>[4x]MGRELSFFLQKESAGFFLGMDAPAGSSVACG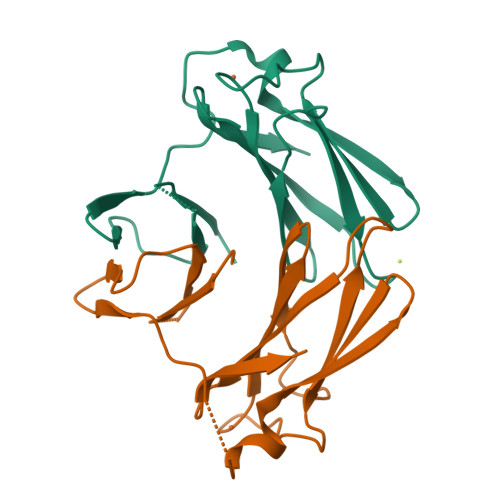SEVLRAVPVGTVDAAKEKHIPVVEVHGHEVKVKVGSVAHPMTPEHYIAWVCLKTRKGIQLKELPVDGAPEVTFALTADDQVLEAYEFCNLHGVWSGK>[2x]FS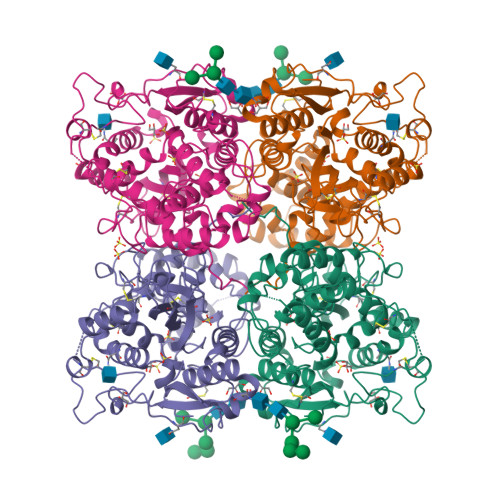YGAAIPQSTQEKQFSQEFRDGYSILKHYGGNGPYSERVSYGIARDPPTSCEVDQVIMVKRHGERYPSPSAGKDIEEALAKVYSINTTEYKGDLAFLNDWTYYVPNECYYNAETTSGPYAGLLDAYNHGNDYKARYGHLWNGETVVPFFSSGYGRVIETARKFGEGFFGYNYSTNAALNIISESEVMGADSLTPTCDTDNDQTTCDNLTYQLPQFKVAAARLNSQNPGMNLTASDVYNLMVMASFELNARPFSNWINAFTQDEWVSFGYVEDLNYYYCAGPGDKNMAAVGAVYANASLTLLNQGPKEAGSLFFNFAHDTNITPILAALGVLIPNEDLPLDRVAFGNPYSIGNIVPMGGHLTIERLSCQATALSDEGTYVRLVLNEAVLPFNDCTSGPGYSCPLANYTSILNKNLPDYTTTCNVSASYPQYLSFWWNYNTTTELNYRSSPIACQEGDAMD> MP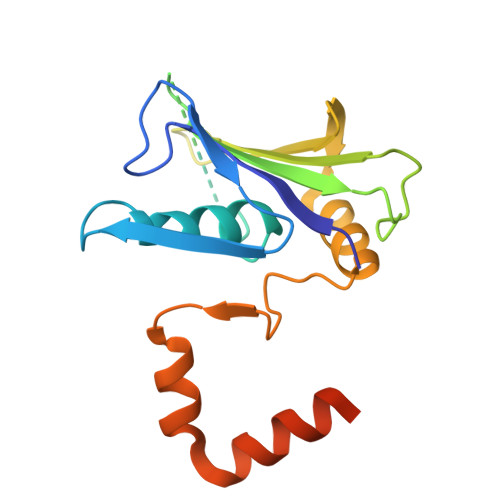YIEKLELKGFKSYGNKKVVIPFSKGFTAIVGANGSGKSNIGDAILFVLGGLSAKAMRASRISDLIFAGSKNEPPAKYAEVAIYFNNEDRGFPIDEDEVVIRRRVYPDGRSSYWLNGRRATRSEILDILTAAMISPDGYNIVLQGDITKFIKMSPLERRLLIDDISGIAEYDSKKEKALEE>EQARPADDALAALGAQLFVDPALSRNATQSCATCHDPARAFTDPREGKAGLAVSVGDDGQSHGDRNTPTLGYAALVPAFHRDANGKYKGGQFWDGRADDLKQQAGQPMLNPVEMAMPDRAAVAARLRDDPAYRTGFEALFGKGVLDDPERAFDAAAEALAAYQATGEFSPFDSKYDRVMRGEEKFTPLEEFGYTVFITWNCRLCHMQRKQGVAERETFTNFEYHNIGLPVNETAREASGLGADHVDHGLLARPGIEDPAQSGRFKVPSLRNVAVTGPYMHNGVFTDLRTAILFYNKYTSRRPEAKINPETGAPWGEPEVARNLSLAELQSGLMLDDGRVDALVAFLETLTDRRYEPLLEESRAAQKDHHHHHH[2x];>ADAPAGTDPRAKWVPQDNDIQACDYWRHCSIDGNICDCSGGSLTNCPPGTKLATASWVASCYNPTDGQSYLIAYRDCCGYNVSGRCPCLNTEGELPVYRPEFANDIIWCFGAEDDAMTYHCTISPIVGKASHHHHHH[2x];>[2x]DAPEAETQAQETQGQAAARAAAADLAAGQDDEPRILEAPAPDARRVYVNDPAHFAAVTQQFVIDGEAGRVIGMIDGGFLPNPVVADDGSFIAHASTVFSRIARGERTDYVEVFDPVTLLPTADIELPDAPRFLVGTYPWMTSLTPDGKTLLFYQFSPAPAVGVVDLEGKAFKRMLDVPDCYHIFPTAPDTFFMHCRDGSLAKVAFGT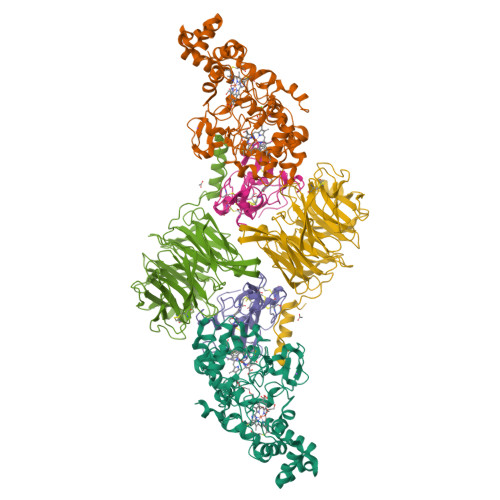EGTPEITHTEVFHPEDEFLINHPAYSQKAGRLVWPTYTGKIHQIDLSSGDAKFLPAVEALTEAERADGWRPGGWQQVAYHRALDRIYLLVDQRDEWRHKTASRFVVVLDAKTGERLAKFEMGHEIDSINVSQDEKPLLYALSTGDKTLYIHDAESGEELRSVNQLGHGPQVITTADMG> GTSSMADIGSRYSKISDNYSSLLQVSEALGRAGLESSNLIVGIDFTKSNEWTGAKSFNRKSLHHLSNTPNPYEQAITIIGRTLAAFDEDNLIPCYGFGDASTHDQDVFSFYPEGRFCNGFEEVLARYREIVPQLKLAGPTSFAPIIEMAMTVVEQSSGQYHVLVIIADGQVTRSVDTEHGRLSPQEQKTVDAIVKASTLPLSIVLVGVGDGPWDMMQEFADNIPARAFDNFQFVNFTEIMSKNKDQSRKETEFALSALMAIPPQYKATIELNLLGVRNGNIPQR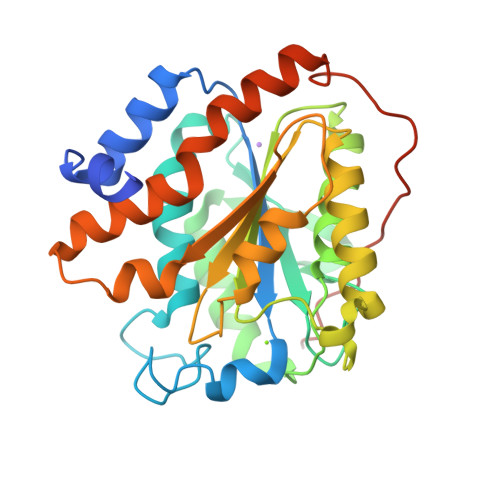IPLPPPVQSGSSFSSSR>MEDVEIKPRGYQLRLVDHLTKSNGIVYLPTGSGKTFVAILVLKRFSQDFDKPIESGGKRALFMCNTVELARQQAMAVRRCTNFKVGFYVGEQGVDDWTRGMWSDEIKKNQVLVGTAQVFLDMVTQTYVALSSLSVVIIDECHHGTGHHPFREFMRLFTIANQTKLPRVVGLTGVLIKGNEITNVATKLKELEITYRGNIITVSDTKEMENVMLYATKPTEVMVSFPHQEQVLTVTRLISAEIEKFYVSLDLMNIGVQPIRRSKSLQCLRDPSKKSFVKQLFNDFLYQMKEYGIYAASIAIISLIVEFDIKRRQAETLSVKLMHRTALTLCEKIRHLLVQKLQDMTYDDDDDNVNTEEVIMNFSTPKVQRFLMSLKVSFADKDPKDICCLVFVERRYTCKCIYGLLLNYIQSTPELRNVLTPQFMVGRNNISPDFESVLERKWQKSAIQQFRDGNANLMICSSVLEEGIDVQACN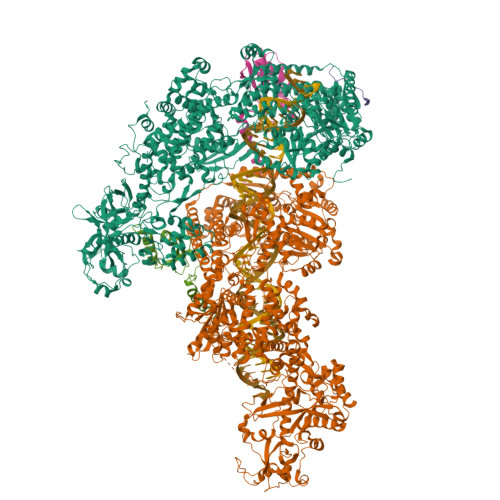HVFILDPVKTFNMYVQSKGRARTTEAKFVLFTADKEREKTIQQIYQYRKAHNDIAEYLKDRVLEKTEPELYEIKGHFQDDIDPFTNENGAVLLPNNALAILHRYCQTIPTDAFGFVIPWFHVLQEDERDRIFGVSAKGKHVISINMPVNCMLRDTIYSDPMDNVKTAKISAAFKACKVLYSLGELNERFVPKTLKERVASIADVHFEHWNKYGDSVTATVNKADKSKDRTYKTECPLEFYDALPRVGEICYAYEIFLEPQFESCEYTEHMYLNLQTPRNYAILLRNKLPRLAEMPLFSNQGKLHVRVANAPLEVIIQNSEQLELLHQFHGMVFRDILKIWHPFFVLDRRSKENSYLVVPLILGAGEQKCFDWELMTNFRRLPQSHGSNVQQREQQPAPRPEDFEGKIVTQWYANYDKPMLVTKVHRELTPLSYMEKNQQDKTYYEFTMSKYGNRIGDVVHKDKFMIEVRDLTEQLTFYVHNRGKFNAKSKAKMKVILIPELCFNFNFPGDLWLKLIFLPSILNRMYFLLHAEALRKRFNTYLNLHLLPFNGTDYMPRPLEIDYSLKRNVDPLGNVIPTEDIEEPKSLLEPMPTKSIEASVANLEITEFENPWQKYMEPVDLSRNLLSTYPVELDYYYHFSVGNVCEMNEMDFEDKEYWAKNQFHMPTGNIYGNRTPAKTNANVPALMPSKPTVRGKVKPLLILQKTVSKEHITPAEQGEFLAAITASSAADVFDMERLEILGNSFLKLSATLYLASKYSDWNEGTLTEVKSKLVSNRNLLFCLIDADIPKTLNTIQFTPRYTWLPPGISLPHNVLALWRENPEFAKIIGPHNLRDLALGDEESLVKGNCSDINYNRFVEGCRANGQSFYAGADFSSEVNFCVGLVTIPNKVIADTLEALLGVIVKNYGLQHAFKMLEYFKICRADIDKPLTQLLNLELGGKKMRANVNTTEIDGFLINHYYLEKNLGYTFKDRRYLLQALTHPSYPTNRITGSYQELEFIGNAILDFLISAYIFENNTKMNPGALTDLRSALVNNTTLACICVRHRLHFFILAENAKLSEIISKFVNFQESQGHRVTNYVRILLEEADVQPTPLDLDDELDMTELPHANKCISQEAEKGVPPKGEFNMSTNVDVPKALGDVLEALIAAVYLDCRDLQRTWEVIFNLFEPELQEFTRKVPINHIRQLVEHKHAKPVFSSPIVEGETVMVSCQFTCMEKTIKVYGFGSNKDQAKLSAAKHALQQLSKCDA[2x];> MDQENFHGSSLPQQLQNLHIQPQQASPNPVQTGFAPRRHYNNLVGLGNGNAVSGSPVKGAPLGQRHVKLKKEKISAQVAQLSQPGQLQLSDVGDPALAGGSGLQGGVGLMGVILPSDEALKFVSETDANGLAMKTPVSILQELLSRRGITPGYELVQIEGAIHEPTFRFRVSFKDKDTPFTAMGAGRSKKEAKHAAARALIDKLIGAQLPESPSSSAGPSVTGLTVAGSGGDGNANATGGGDASDKTVGNPIGWLQEMCMQRRWPPPSYETETEVGLPHERLFTIACSILNYREMGKGKSKKIAKRLAAHRMWMRLQETPIDSGKISDSICGELEGEVSIIQDIDRYEQVSKDFEFIKI;>[2x]MDNKSAVSALQEFCARTQINLPTYSFIPGEDGGYVCKVELLEIEALGNGRSKRDAKHLAASNILRKIQLLPGIHGLMKDSTVGDLDEELTNLNRDMVKELRDYCVRREMPLPCIEVVQQSGTPSAPEFVACCSVASIVRYGKSDKKKDARQRAAIEMLALISSNSDNLRPDQMQVASTSKLKVVDMEESMEELEALRRKKFTTYWELKEAGSVDHTGMRLCDRHNYFKNFYPTLKKEAIEAINSDEYESSKDKAMDVMSSLKITPKISEVESSSLVPLLSVELNCAFDVVLMAKETDIYDHIIDYFRTMLI> MKVAVLPGDGIGPEVTEAALKVLRALDEAEGLGLAYEVFPFGGAAIDAFGEPFPEPTRKGVEEAEAVLLGSVGGPKWDGLPRKISPETGLLSLRKSQDLFANLRPAKVFPGLERLSPLKEEIARGVDVLIVRELTGGIYFGEPRGMSEAEAWNTERYSKPEVERVARVAFEAARKRRKHVVSVDKANVLEVGEFWRKTVEEVGRGYPDVALEHQYVDAMAMHLVRSPARFDVVVTGNIFGDILSDLASVLPGSLGLLPSASLGR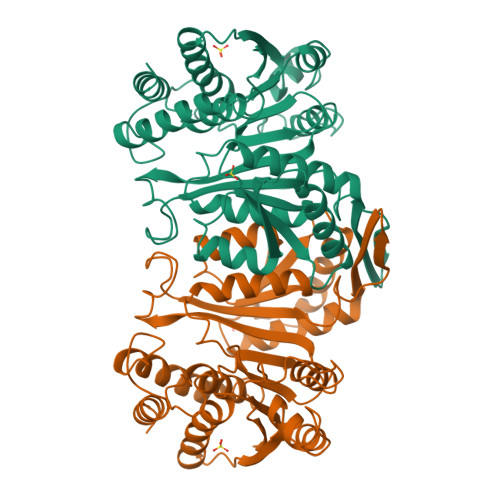GTPVFEPVHGSAPDIAGKGIANPTAAILSAAMMLEHAFGLVELARKVEDAVAKALLETPPPDLGGSAGTEAFTATVLRHLA>GAMEGEEGDDRPREHPFVVTEPGELARGKKNGLDYLFNLYEQAGKFLEEVQHIAREKGEKCPTKVTNQVFRHAKVQGAGYINKPKMRQYVHCYALHCLASDKSDELRRCCKERGENVGAWCQACYLPLIKMAKEKSWDIEGLFNSHDKLKIWYVPKKLIQLCHQEK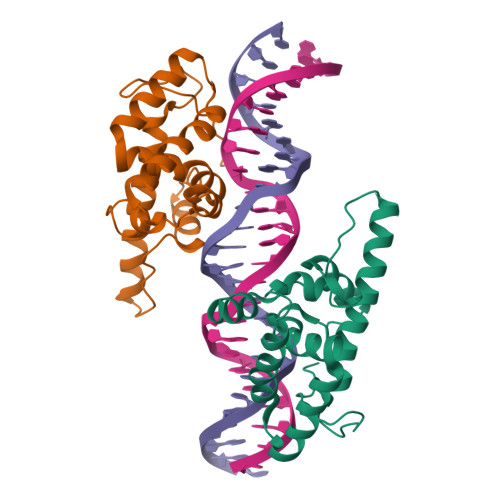SK[2x]(2E,6E)-2,6-dimethylocta-2,6-dienedial 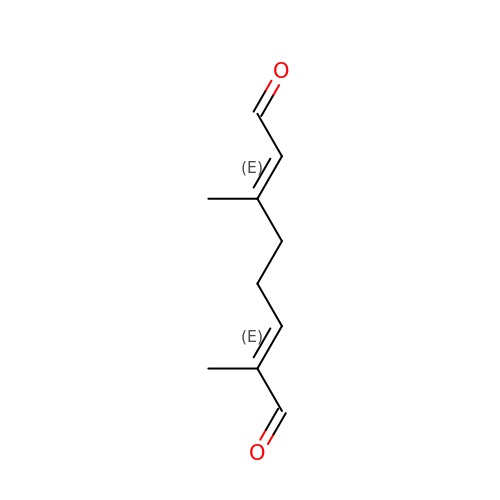| C10 H14 O2 | GRHWFPUCRVCMRY-TXFIJWAUSA-N> AUSAEQVEKLRNKINNAAVLVFAKSFCPYCKKVMERFNNLKIPFGYLDLDLKKNGSDYQKMLQEITGRTTVPQVFFRGEFIGGCDDVMAIDDDTIVKKANEMKYDYDMVIIGGGSGGLALAKESAKSGAKVALLDFVVPTPMGTTWGLGGTCVNVGCIPKKLMHQAALLNHYMEDAKSFGWDVDKGPHDWVKMVEGIQDHIHALNFGYRSSMMNANVKYLNALGEIVDPHTIKTTNKQGIVKNITTNTIIVATGERPRYPPIPGAKEYGITSDDLFTLDHNPGKTLCVGASYVSLECAGFLSSIGCDVTVMVRSIFLRGFDQQMAGLISDYIAKYGVKFVRPCVPTSVRCLEEYDPESGKLAIYEVEGKHEDGTPFKDTFNTVLFAVGRDPCTTNIGLQNVDVKTTNGRVVVDDEERTNVPNIYAIGDVSNAGYQLTPLAIQAGKNLARRLYTADDCRTDYTNVPTTVFTPLEYGCIGLSEENAISKFGEDNIEVFHSYFQPLEWTVPHRPDNTCYAKLIINKQDDNRVVGFHVFGPNAGEVTQGYAVAMHLGARKEDFDRTIGIHPTCSETFTTLRVTKSSGASA;> SAEQVEKLRNKINNAAVLVFAKSFCPYCKKVMERFNNLKIPFGYLDLDLKKNGSDYQKMLQEITGRTTVPQVFFRGEFIGGCDDVMAIDDDTIVKKANEMKYDYDMVIIGGGSGGLALAKESAKSGAKVALLDFVVPTPMGTTWGLGGTCVNVGCIPKKLMHQAALLNHYMEDAKSFGWDVDKGPHDWVKMVEGIQDHIHALNFGYRSSMMNANVKYLNALGEIVDPHTIKTTNKQGIVKNITTNTIIVATGERPRYPPIPGAKEYGITSDDLFTLDHNPGKTLCVGASYVSLECAGFLSSIGCDVTVMVRSIFLRGFDQQMAGLISDYIAKYGVKFVRPCVPTSVRCLEEYDPESGKLAIYEVEGKHEDGTPFKDTFNTVLFAVGRDPCTTNIGLQNV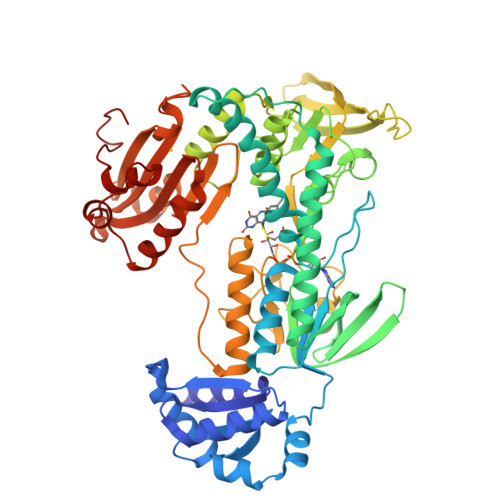DVKTTNGRVVVDDEERTNVPNIYAIGDVSNAGYQLTPLAIQAGKNLARRLYTADDCRTDYTNVPTTVFTPLEYGCIGLSEENAISKFGEDNIEVFHSYFQPLEWTVPHRPDNTCYAKLIINKQDDNRVVGFHVFGPNAGEVTQGYAVAMHLGARKEDFDRTIGIHPTCSETFTTLRVTKSSGASA>[2x]MAQTPAFDKPKVELHVHLDGSIKPETILYYGRRRGIALPANTAEGLLNVIGMDKPLTLPDFLAKFDYYMPAIAGCREAIKRIAYEFVEMKAKEGVVYVEVRYSPHLLANSKVEPIPWNQAEGDLTPDEVVALVGQGLQEGERDFGVK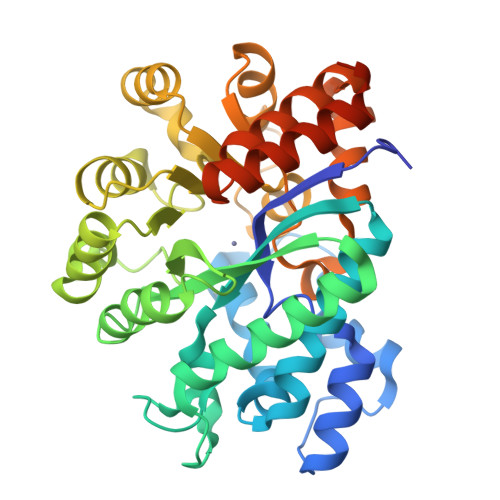ARSILCCMRHQPNWSPKVVELCKKYQQQTVVAIDLAGDETIPGSSLLPGHVQAYQEAVKSGIHRTVHAGEVGSAEVVKEAVDILKTERLGHGYHTLEDQALYNRLRQENMHFEICPWSSYLTGAWKPDTEHAVIRLKNDQANYSLNTDDPLIFKSTLDTDYQMTKRDMGFTEEEFKRLNINAAKSSFLPEDEKRELLDLLYKAYGMPPSASAGQNLENLYFQSGG3-[3-(aminomethyl)phenyl]-~{N}-[(1~{S})-1,2,3,4-tetrahydronaphthalen-1-yl]benzamide 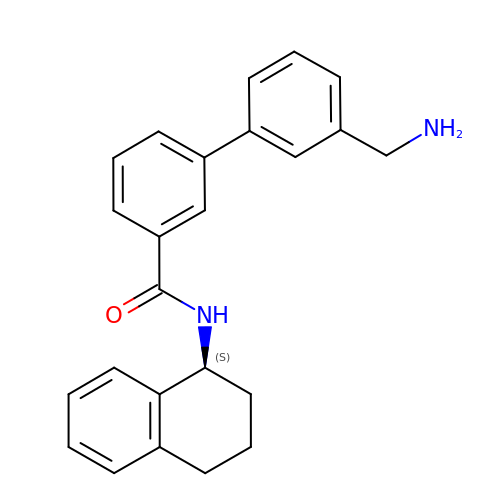| C24 H24 N2 O | ONRUCWPTBOHFGA-QHCPKHFHSA-N>[2x]GSGSMISIFIAEDQQMLLGALGSLLNLEDDMEVVGKGTTGQDAVDFVKKRQPDVCIMDIEMPGKTGLEAAEE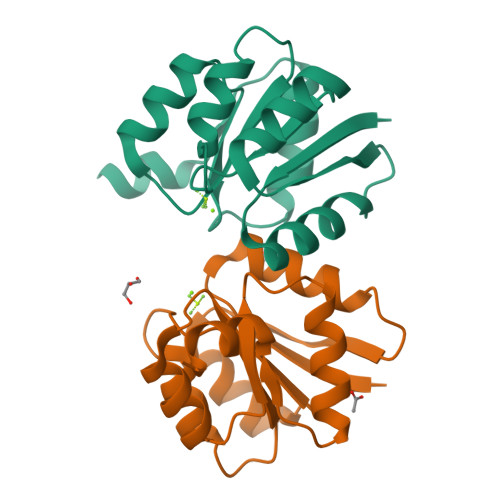LKDTGCKIIILTTFARPGYFQRAIKAGVKGYLLKDSPSEELANAIRSVMNGKRIYAPELMEDLYSEA>GPGSMNIKEIAVGKNPPEDVNVIVEVSLGGQPIKYEMDKKSGALFVDRFL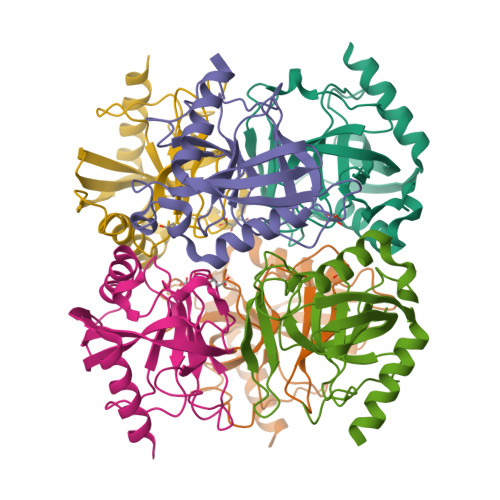YTSMVYPGNYGFVPHTLSEDGDPIDVLICNTRPLLPGCVINVYPIGALIMEDDGGKDEKIIAIPTPKLTQRYNNIHDYTDLPEITLKQIEHFFEHYKDLEPGKWAKIEGWRDKSFAHELIKQAIERNKEL[6x]> MKITCTDLVYVFILLFLNTSCVQAVFSDDAFITDWQLANLGPWEKVIPDSRDRNRVLILSNPTETSCLVSSFNVSSGQILFRNVLPFTIDEIQLDSNDHNAMVCVNSSSNHWQKYDLHDWFLLEEGVDNAPSTTILPQSSYLNDQVSIKNNELHILDEQSKLAEWKLELPQGFNKVEYFHREDPLALVLNVNDTQYMGFSANGTELIPVWQRDEWLTNVVDYAVLDVFDSRDVELNKDMKAELDSNSLWNAYWLRLTTNWNRLINLLKENQFSPGRVFTKLLALDAKDTTVSDLKFGFAKILIVLTHDGFIGGLDMVNKGQLIWKLDLEIDQGVKMFWTDKNHDELVVFSHDGHYLTIEVTKDQPIIKSRSPLSERKTVDSVIRLNEHDHQYLIKFEDKDHLLFKLNPGKNTDVPIVANNHSSSHIFVTEHDTNGIYGYIIENDTVKQTWKKAVNSKEKMVAYSKRETTNLNTLGITLGDKSVLYKYLYPNLAAYLIANEEHHTITFNLIDTITGEILITQEHKDSPDFRFPMDIVFGEYWVVYSYFSSEPVPEQKLVVVELYESLTPDERLSNSSDNFSYDPLTGHINKPQFQTKQFIFPEIIKTMSISKTTDDITTKAIVMELENGQITYIPKLLLNARGKPAEEMAKDKKKEFMATPYTPVIPINDNFIITHFRNLLPGSDSQLISIPTNLESTSIICDLGLDVFCTRITPSGQFDLMSPTFEKGKLLITIFVLLVITYFIRPS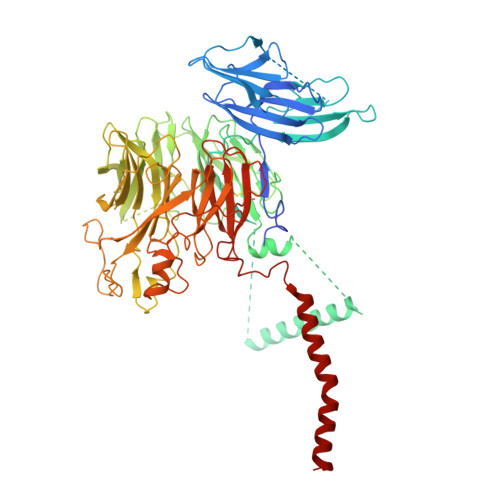VSNKKLKSQWLIK> MKDDLDNNLLYRYCGATSPFWRLPLDSNALQLAASEEAVTSHVVPLTPEQAAQIRTMSVITSSVTLSLS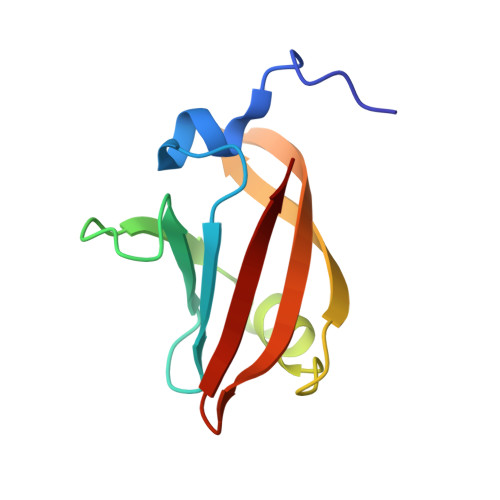LFGELVPVHLVGRKVSRKEWAGTASA>MLKLQTLQALICIEEVGSLRAAAQLLHLSQPALSAAIQQLEDELKAPLLVRTKRGVSLTSFGQAFMKHARLIVTESRRAQEEIGQLRGRWEGHITFAASPAIALAALPLALASFAREFPDVTVNVRDGMYPAVSPQLRDGTLDFALTAAHKHDIDTDLEAQPLYVSDVVIVGQRQHPMANATRLAELQECRWAFSSAPRGPGAIIRNAFARYGLPEPKLGLVCESFLALPGVVAHSDLLTTMPRTLYERNAFKDQLCSIPLQDALPNPTIYVLRRHDLPVTPAAAGLIRW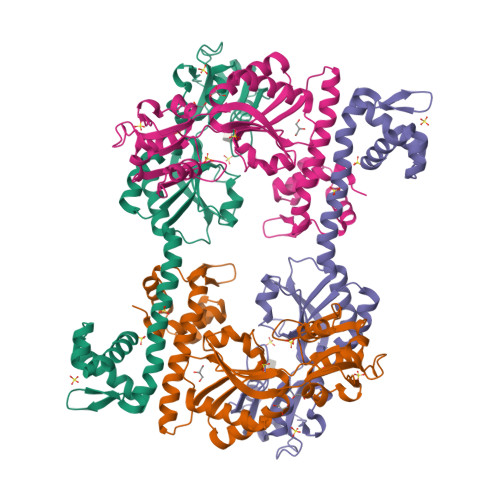IQHHALQTGHHHHHH[2x]> GPGIWLREVDRDKLIAVAKKLKEIIPDR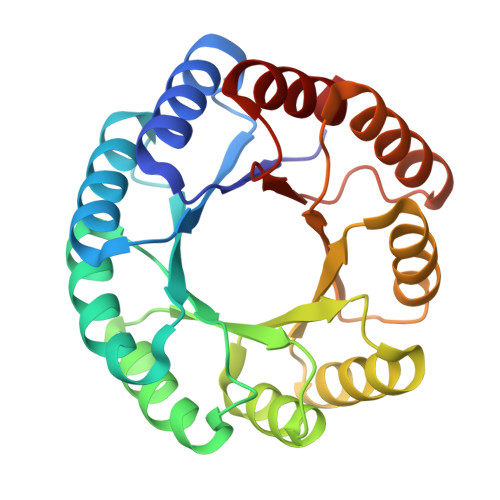VKGFVVGGKTDDVVATIRDLIALFGPDLEIVVELTELDKAIETMKKAVEAGASAILLRDGVRGVEELRKIAEEAKKLGVKVIVDVTDGPDVLELAREAAALADAIVIDTGLPLDTREAIAALADAAGVDVIFRVSGLDQVDDAVALAARTPAFKGFLLEGVRDVAAAEAVRARLAAAGLTDLDFLLALDGLDVDTAIAAALALLE>MGHHHHHHEFMHVFDNNGIELKAECSIGEEDGVYGLILESWGPGDRNKDYNIALDYIIERLVDSGVSQVVVY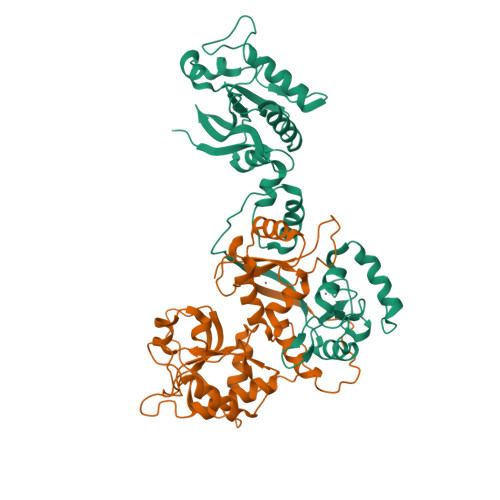LASSSVRKHMHSLDERKIHPGEYFTLIGNSPRDIRLKMCGYQAYFSRTGRKEIPSGNRTKRILINVPGIYSDSFWASIIRGELSELSQPTDDESLLNMRVSKLIKKTLSQPEGSRKPVEVERLQKVYVRDPMVEAWILQQSKGICENCGKNAPFYLNDGNPYLEVHHVIPLSSGGADTTDNCVALCPNCHRELHYSKNAKELIEMLYVNINRLQK[2x]> SNAERIIHGDVLSPILAYMRLKGQHKVILESIPRDKETARFSILAYNPVFEIKFENGVLYQNGQVIDRDPLDFLYEVIHKSQHHSELPFGGGAIGFVGYDMISLYEEIGQIPEDTIGTPDMHFFVYESYMVFDHKKEKIHVIEDALYSERSQEALEKSLNQVLEELRIPAPNEFEDLDLSPLDFKPHIAPHKFEGMVETARDLIRNGDMFQCVLSQRFSAEVTGNPFDFYRNLRVTNPSN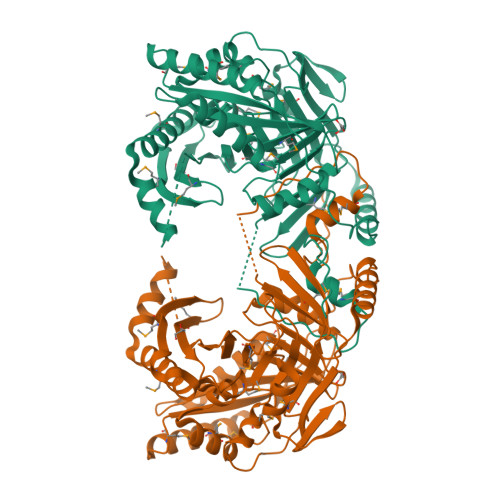YLYFYDFGDYQIIGASPESLVSVKNGIVTTNPIAGTRPRGATDEEDKALATDLLSDEKETAEHRMLVDLGRNDIGRISETTSVQVTKYMEVELFRYVMHLTSVVKGRLLPELTAMDALKATLPAGTVSGAPKIRAMRRIYELETEKRGVYAGAIGYLSATGDMDLAIAIRTMILKNQRAYVQAGAGIVYDSIAQNEYQETINKAKSMTRI>MASMTGMPNYNIPFSPPDITEAEITEVVDTLRSGWITTGPKTKELERRLSLYTQTPKTVCLNSATAALELILRVLEVGPGDEVIVPAMTYTASCSVITHVGATPVMVDIQADTFEMDYDLLEQAITEKTKVIIPVELAGIVCDYDRLFQVVEKKRDFFTASSKWQKAFNRIVIVSDSAHALGSTYKGQPSGSIADFTSFSFHAVKNFTTAEGGSATWKANPVIDDEEMYKEFQILSLHGQTKDALAKMQLGSWEYDIVTPAYKCNMTDIMASLGLVQLDRYPSLLQRRKDIVDRYDSGFAGSRIHPLAHKTETVESSRHLYITR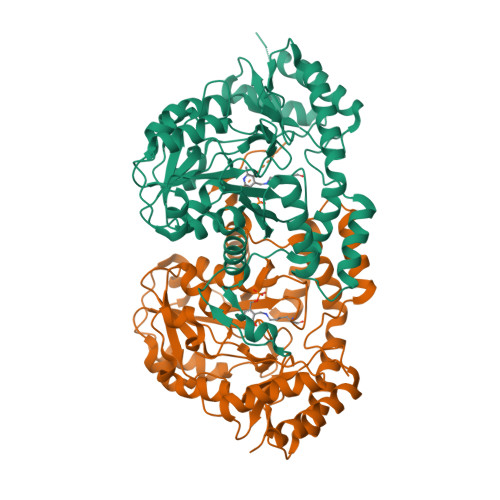VEGASLEERNLIIQELAKAGIASNVHYKPLPLLTAYKNLGFDMTNYPKAYAFFENEITLPLHTKLSDEEVDYIIETFKTVSEKVLTLSKKKLAAALEHHHHHH[4x]4-[[4-[(4-azanyl-1-methyl-pyrrol-2-yl)carbonylamino]-1-methyl-pyrrol-2-yl]carbonylamino]-~{N}-[2-[[(3~{S})-3-azanyl-4-oxidanylidene-butyl]carbamoyl]-1-methyl-imidazol-4-yl]-1-methyl-imidazole-2-carboxamide 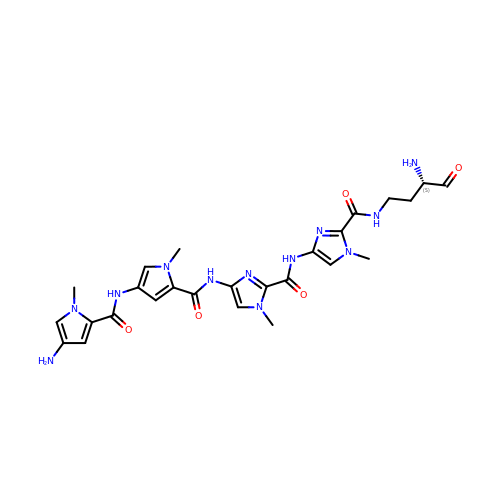| C26 H32 N12 O5 | UZFBAFZKKPMVCV-AWEZNQCLSA-N>[2x]ADALHIRFPDGAVIEYEPETSALTVSGIKTASVTASGSVTATVPVVMVKASTRVTLD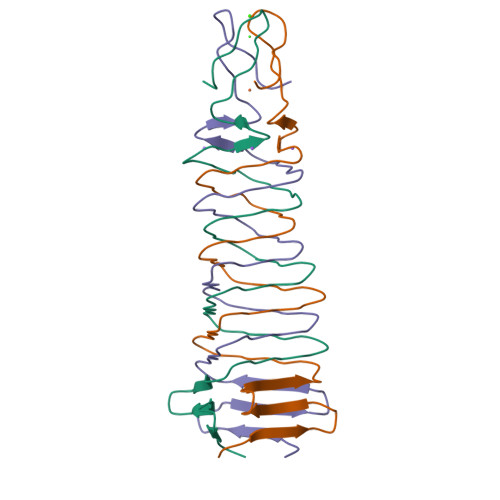TPEVVCTNRLITGTLEVQKGGTMRGNIEHTGGELSSNGKVLHTHKHPGDSGGTTGSPL>[7x]MGSSHHHHHHSGQHAVSAYLADARRALGSAGCSQLLAALTAYKQDDDLDKVLAVLAAL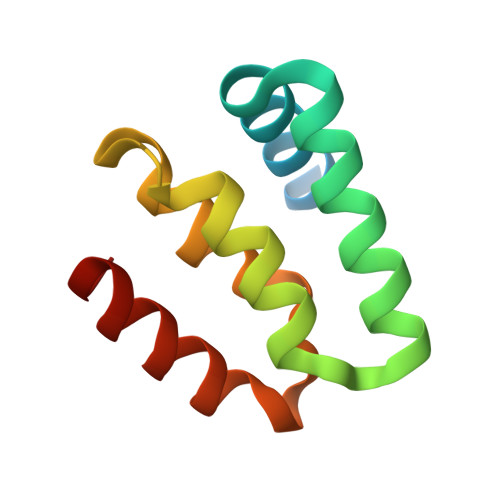TTAKPEDFPLLHRFSMFVRPHHKQRFSQTCTDLTGRPY>[2x]ARDPKHDILFEPIQIGPKTLRNRFYQVPHAIGAGSDKPGFQSAHRSV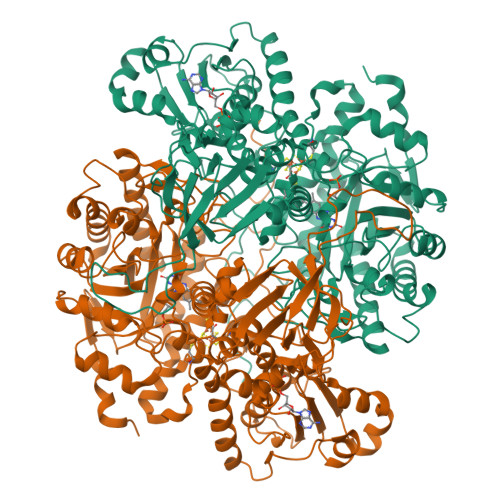KAEGGWAALNTEYCSINPESDDTHRLSARIWDEGDVRNLKAMTDEVHKYGALAGVELWYGGAHAPNMESRATPRGPSQYASEFETLSYCKEMDLSDIAQVQQFYVDAAKRSRDAGFDIVYVYGAHSYLPLQFLNPYYNKRTDKYGGSLENRARFWLETLEKVKHAVGSDCAIATRFGVDTVYGPGQIEAEVDGQKFVEMADSLVDMWDITIGDIAEWGEDAGPSRFYQQGHTIPWVKLVKQVSKKPVLGVGRYTDPEKMIEIVTKGYADIIGCARPSIADPFLPQKVEQGRYDDIRVCIGCNVCISRWEIGGPPMICTQNATAGEEYRRGWHPEKFRQTKNKDSVLIVGAGPSGSEAARVLMESGYTVHLTDTAEKIGGHLNQVAALPGLGEWSYHRDYRETQITKLLKKNKESQLALGQKPMTADDVLQYGADKVIIATGARWNTDGTNCLTHDPIPGADASLPDQLTPEQVMDGKKKIGKRVVILNADTYFMAPSLAEKLATAGHEVTIVSGVHLANYMHFTLEYPNMMRRLHELHVEELGDHFCSRIEPGRMEIYNIWGDGSKRTYRGPGVSPRDANTSHRWIEFDSLVLVTGRHSECTLWNELKARESEWAENDIKGIYLIGDAEAPRLIADATFTGHRVAREIEEANPQIAIPYKRETIAWGTPHMPGGNFKIEYKV> EKWMEIDVLKQKVAKSSDMAFAISSEHEKYLWTKMGCLVPIQVKWKLDKRHFNSNLSLRIRFVKYDKKENVEYAIRNPRSDVMKCRSHTEREQHFPFDSFFYIRNSEHEFSYSAEKGSTFTLIMYPGAVQANFDIIFMCQEKCLDLDDRRKT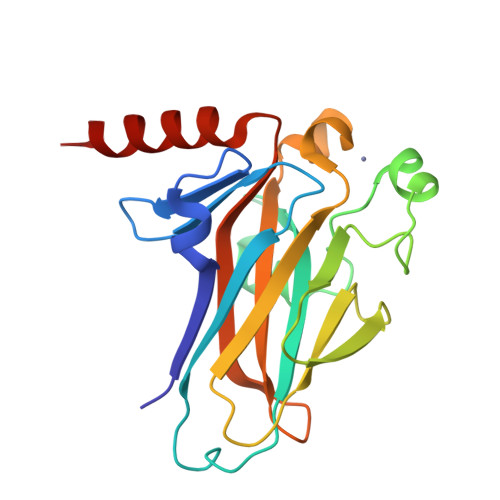MCLAVFLDDENGNEILHAYIKQVRIVAYPRRDWKNFCEREDAKQ>GDTLGASWHRPDKCCLGYQKRPLPQVLLSSWYPTSQLCSKPGVIFLTKRGRQVCADKSKDWVK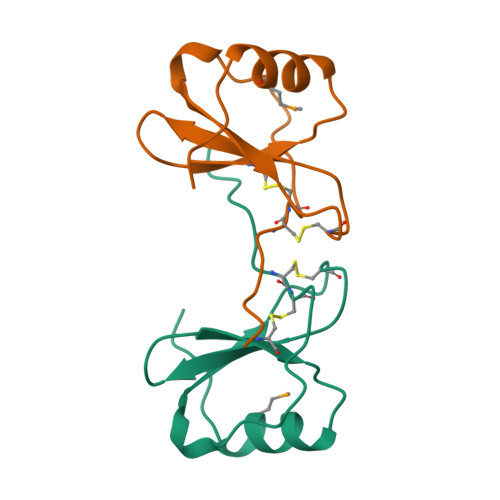KLMQQLPVTAR[2x]> MTTTMKISIEFLEPFRMTKWQESTRRNKNNKEFVRGQAFARWHRNKKDNTKGRPYITGTLLRSAVIRSAENLLTLSDGKISEKTCCPGKFDTEDKDRLLQLRQRSTLRWTDKNPCPDNAETYCPFCELLGRSGNDGKKAEKKDWRFRIHFGNLSLPGKPDFDGPKAIGSQRVLNRVDFKSGKAHDFFKAYEVDHTRFPRFEGEITIDNKVSAEARKLLCDSLKFTDRLCGALCVIRFDEYTPAADSGKQTENVQAEPNANLAEKTAEQIISILDDNKKTEYTRLLADAIRSLRRSSKLVAGLPKDHDGKDDHYLWDIGKKKKDENSVTIRQILTTSADTKELKNAGKWREFCEKLGEALYLKSKDMSGGLKITRRILGDAEFHGKPDRLEKSRSVSIGSVLKETVVCGELVAKTPFFFGAIDEDAKQTALQVLLTPDNKYRLPRSAVRGILRRDLQTYFDSPCNAELGGRPCMCKTCRIMRGITVMDARSEYNAPPEIRHRTRINPFTGTVAEGALFNMEVAPEGIVFPFQLRYRGSEDGLPDALKTVLKWWAEGQAFMSGAASTGKGRFRMENAKYETLDLSDENQRNDYLKNWGWRDEKGLEELKKRLNSGLPEPGNYRDPKWHEINVSIEMASPFINGDPIRAAVDKRGTAVVTFVKYKAEGEEAKPVCAYKAESFRGVIRSAVARIHMEDGVPLTELTHSDCECLLCQIFGSEYEAGKIRFEDLVFESDPEPVTFDHVAIDRFTGGAADKKKFDDSPLPGSPARPLMLKGSFWIRRDVLEDEEYCKALGKALADVNNGLYPLGGKSAIGYGQVKSLGIKGDDKRISRLMNPAFDETDVAVPEKPKTDAEVRIEAEKVYYPHYFVEPHKKVEREEKPCGHQKFHEGRLTGKIRCKLITKTPLIVPDTSNDDFFRPADKEARKEKDEYHKSYAFFRLHKQIMIPGSELRGMVSSVYETVTNSCFRIFDETKRLSWRMDADHQNVLQDFLPGRVTADGKHIQKFSETARVPFYDKTQKHFDILDEQEIAGEKPVRMWVKRFIKRLSLVDPAKHPQKKQDNKWKRRKEGIATFIEQKNGSYYFNVVTNNGCTSFHLWHKPDNFDQEKLEGIQNGEKLDCWVRDSRYQKAFQEIPENDPDGWECKEGYLHVVGPSKVEFSDKKGDVINNFQGTLPSVPNDWKTIRTNDFKNRKRKNEPVFCCEDDKGNYYTMAKYCETFFFDLKENEEYEIPEKARIKYKELLRVYNNNPQAVPESVFQSRVARENVEKLKSGDLVYFKHNEKYVEDIVPVRISRTVDDRMIGKRMSADLRPCHGDWVEDGDLSALNAYPEKRLLLRHPKGLCPACRLFGTGSYKGRVRFGFASLENDPEWLIPGKNPGDPFHGGPVMLSLLERPRPTWSIPGSDNKFKVPGRKFYVHHHAWKTIKDGNHPTTGKAIEQSPNNRTVEALAGGNSFSFEIAFENLKEWELGLLIHSLQLEKGLAHKLGMAKSMGFGSVEIDVESVRLRKDWKQWRNGNSEIPNWLGKGFAKLKEWFRDELDFIENLKKLLWFPEGDQAPRVCYPMLRKKDDPNGNSGYEELKDGEFKKEDRQKKLTTPWTPWA;> MSNPIRDIQDRLKTAKFDNKDDMMNLASSLYKYEKQLMDSSEATLCQQGLSNRPNSFSQLSQFRDSDIQSKAGGQTGKFWQNEYEACKNFQTHKERRETLEQIIRFLQNGAEEKDADDLLLKTLARAYFHRGLLYRPKGFSVPARKVEAMKKAIAYCEIILDKNEEESEALRIWLYAAMELRRCGEEYPENFAEKLFYLANDGFISELYDIRLFLEYTEREEDNNFLDMILQENQDRERLFELCLYKARACFHLNQLNDVRIYGESAIDNAPGAFADPFWDELVEFIRMLRNKKSELWKEIAIKAWDKCREKEMKVGNNIYLSWYWARQRELYDLAFMAQDGIEKKTRIADSLKSRTTLRIQELNELRKDAHRKQNRRLEDKLDRIIEQENEARDGAYLRRNPPCFTGGKREEIPFARLPQNWIAVHFYLNELESHEGGKGGHALIYDPQKAEKDQWQDKSFDYKELHRKFLEWQENYILNEEGSADFLVTLCREIEKAMPFLFKSEVIPEDRPVLWIPHGFLHRLPLHAAMKSGNNSNIEIFWERHASRYLPAWHLFDPAPY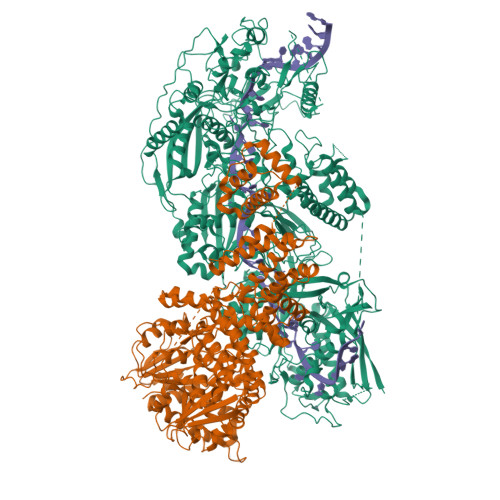SREESSTLLKNFEEYDFQNLENGEIEVYAPSSPKKVKEAIRENPAILLLLCHGEADMTNPFRSCLKLKNKDMTIFDLLTVEDVRLSGSRILLGACESDMVPPLEFSVDEHLSVSGAFLSHKAGEIVAGLWTVDSEKVDECYSYLVEEKDFLRNLQEWQMAETENFRSENDSSLFYKIAPFRIIGFPAE4-(1,3-BENZODIOXOL-5-YLOXY)-2-[4-(1H-IMIDAZOL-1-YL)PHENOXY]PYRIMIDINE 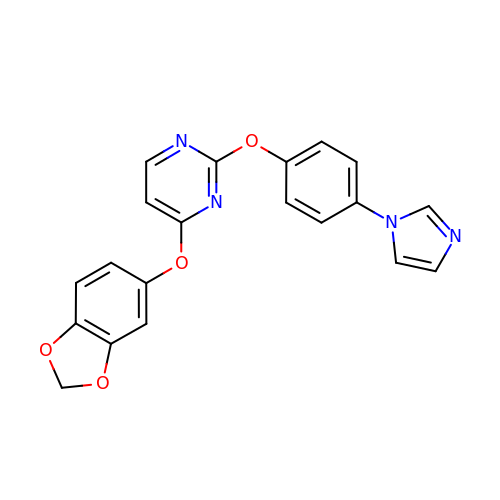| C20 H14 N4 O4 | XPXGYINSBORUMM-UHFFFAOYSA-N> IWGIGCNPWTA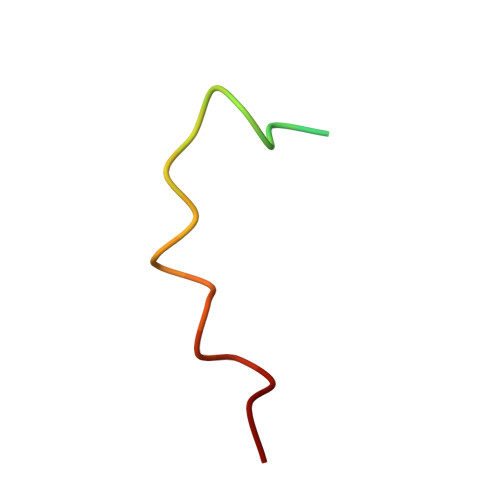EHVDQTLASGNDIC>[6x]GSKPLAEQDWYHGAIPRIEAQELLKK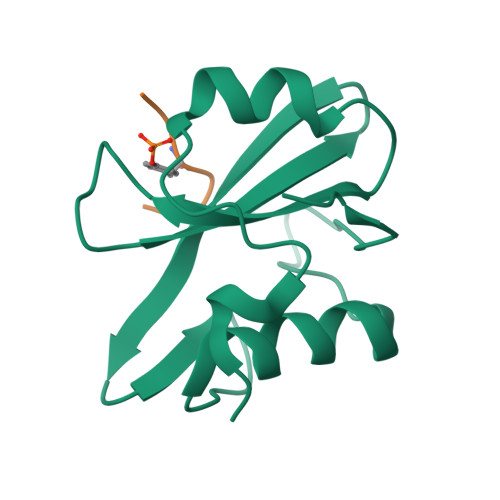QGDFLVRESHGKPGEYVLSVYSDGQRRHFIIQYVDNMYRFEGTGFSNIPQLIDHHYTTKQVITKKSGVVLLNPIPK;>DEYENVD[6x]>[2x]TIPDAMIVIDGHGIIQLFSTAAERL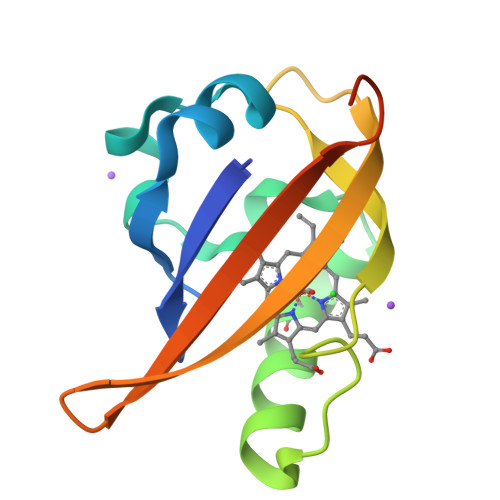FGWSELEAIGQNVNILMPEPDRSRHDSYISRYRTTSDPHIIGIGRIVTGKRRDGTTFPMHLSIGEMQSGGEPYFTGFVRDLTEHQQTQARLQEL>[2x]DLSQCDREPIHLLGGIQSHGVLLAFRGPDRLLEVVSANAQALLGRPPETLLGQPVGRVLPAEVLAQWEPLVARGSVRVVLPAGAYRALLHESDGLTVLELEPAELQPDMEETALEVVRRLVSPLAGVKGTQALLQTAADTVRALTGFDRVMVYRFDADWHGEVLAESKRGGMDGFLGMHFPATDIPVQARALYTRNPLRLIADARARPVPLLPPVVPALGRPLDLSNSALRSVSPVHLEYLRNMGVGASFSLSLLKEGVLWGLIACHHLEPLHISHERRRACEVLTQLLALQLSAEER

Phytochromes are red-light photoreceptors first identified in plants, with homologs found in bacteria and fungi, that regulate a variety of critical physiological processes. They undergo a reversible photocycle between two distinct states: a red-light-absorbing Pr form and a far-red light-absorbing Pfr form. BphPs exist as dimers where each strand of amino acids has the same chemical composition (sequence). BphPs consist of a photosensory core module (PCM) and an output effector module (OM) [Fig. 1(a)]. The PCM consists of three domains: PAS (Per-Arndt-Sim), GAF (cGMP phosphodiesterase/adenylyl cyclase/FhIA), and PHY (phytochrome-specific GAF-related). The central chromophore, biliverdin (BV) [Fig. 1(b)], is a heme-derived open-chain tetrapyrrole (consisting of pyrrole rings A–D) which is covalently bound via its 3″ position to a conserved N-terminal cysteine (Cys13).

In addition, we demonstrate how crystals of a severely truncated fragment of SaBphP2 can be obtained from which an x-ray structure with a very unusual chromophore configuration is determined. The overall structure of the fragment differs from those of the CBD of SaBphP1 and the CBD part of the SaBphP2 PCM. The asymmetric unit harbors a dimer (dimer-NCS) where the subunits are related by non-crystallographic symmetry (NCS) [Fig. 5(a)]. Subunits in the dimer-NCS interact much differently than in the CBDs of the other constructs. A dimer of dimers (dimer-SYM) is formed through crystallographic symmetry [Fig. 5(b)]. However, the angle between the interface helices is about 90° rather than around 35° as observed for the other constructs mentioned. The interfaces of both the dimer-NCS and the dimer-SYM are very different from those normally observed in CBD and PCMs of BphPs. The most notable difference to all other phytochromes, however, is the structure of the BV chromophore. Rather being in a stretched-out (all-Z) syn–syn–anti configuration, the BV assumes a curved all-Z, all-syn configuration [Fig. 6(a)], which has never been observed so far. However, BV cannot close to heme again, as this requires a reduction reaction. Consequently, ring-D is stacked on top of ring A, and the BV forms a spiral staircase [with the pyrrole rings as four steps, Fig. 6(a)] in both subunits. Nevertheless, the fragmentation results in an interesting chromophore configuration and large amino acid displacements that were never seen before in phytochromes and that could even be transiently occupied at some stage in the photocycle.> MSSERVFHLCVCSPLDSILTSQIYNHIEQIAPNIHVMFKSSLNQNTEHQLRYQETEFVISYEDFHRPEFTSVPLFKDEMVLVASKNHPTIKGPLLKHDVYNEQHAAVSLDRFASFSQPWYDTVDKQASIAYQGMAMMSVLSVV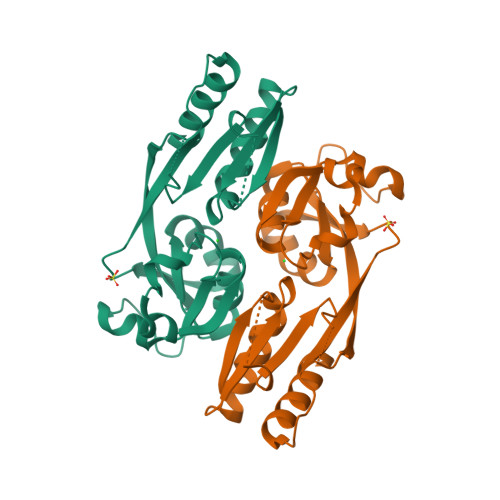SQTHLVAIAPRWLAEEFAESLELQVLPLPLKQNSRTCYLSWHEAAGRDKGHQWMEEQLVSICKRLEHHHHHH> IAELPPKVSVFVPPRDGFFGNPRKSKLICQATGFSPRQIQVSWLREGKQVGSGVTTDQVQAEAKESGPTTYKVTSTLTIKESDWLGQSMFTCRVDHRGLTFQQNASSMCVPDQDTAIRVFAIPPSFASIFLTKSTKLTCLVTDLTTYDSVTISWTRQNGEAVKTHTNISESHPNATFSAVGEASICEDDWNSGERFTCTVTHTDLPSPLKQTISRPKGVALHRPDVYLLPPAREQLNLRESATITCLVTGFSPADVFVQWMQRGQPLSPEKYVTSAPMPEPQAPGRYFAHSILTVSEEEWN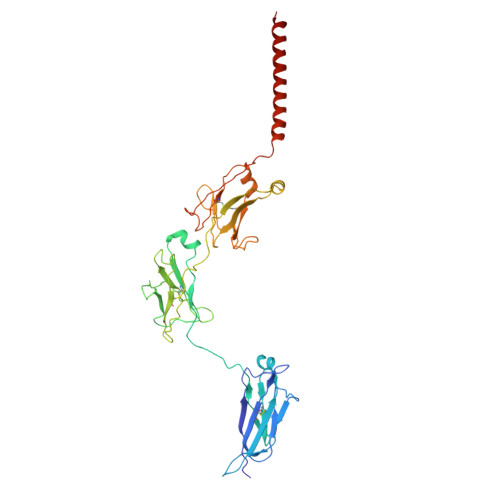TGETYTCVVAHEALPNRVTERTVDKSTEGEVSADEEGFENLWATASTFIVLFLLSLFYSTTVTLFK> SHHHHHHSSGLVPRGSHMTSSNDISLASKDPTTFPLGCSPDITTPKKGLSMELYSYDFRKKGSYPCWDAAYLDPNYPRTGYKSHRLL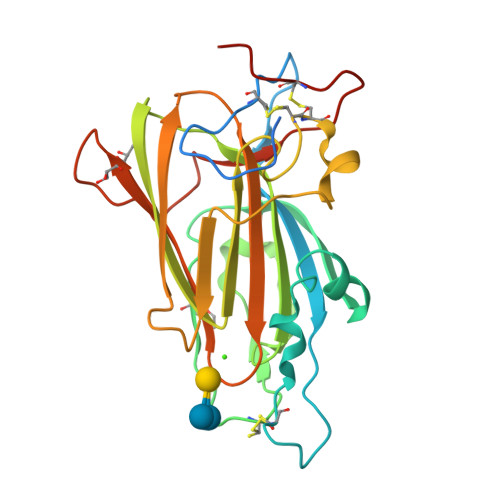AKVDGVTGNINFYYHATKGCTPQLGHLPASYNYPKPLTMTNFTMLLYGYFRPKVTGFHTFTISADDLLFVNFGAGNAFDCCRRDSSADHFGNYQAYAIWGSKTAKDELTVHLDAGVYYPIRLFYNNRDNDGALSFTFKTESNENTVSDFSEYFFSLDDTEEGCPGLISYDSS>GPGSAVPFVEDWRLVQTLGEGAYGEVQLAVNRVTEEAVAVKIVDMKRAVDCPENIKKEICINKMLNHENVVKFYGHRREGNIQYLFLEYCSGGELFDRIEPDIGMPEPDAQRFFHQLMAGVVYLHGIGITHRDIKPENLLLDERDNLKISDFGLATVFRYNNRERLLNKMCGTLPYVAPELLKRREFHAEPVDVWSCGIVLTAMLAGELPWDQPSDSCQEYSDWKEKKTYLNPWKKIDSAPLALLHKILVENPSARITIPDIKKDRWYNKPLKKGAKR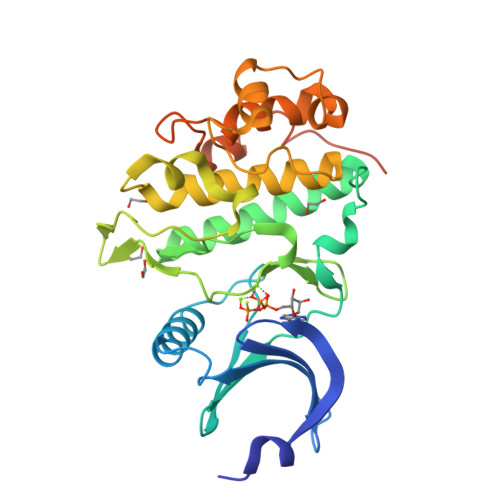PRVTSGGVSESPHHHHHHHH[2x]2-amino-N-(4-methyl-1,3-thiazol-2-yl)-5-[(4-methyl-4H-1,2,4-triazol-3-yl)sulfanyl]benzamide 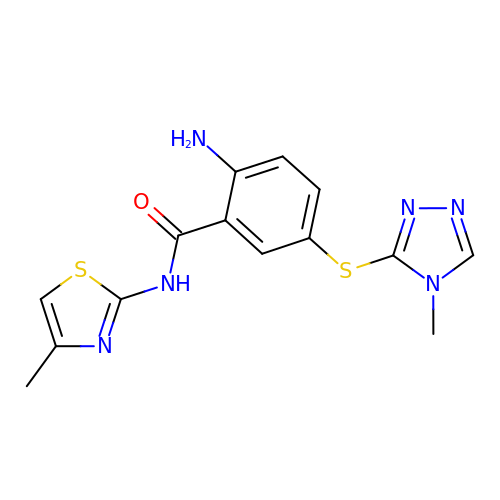| C14 H14 N6 O S2 | JEBOJMQHVUEKBE-UHFFFAOYSA-N> SDWISFSHMSSDTDHFPIKSWFRCEQKAASRSYATLGDMSHPQGIYEVRAAITRLISLTRGVKCRPEQMIIGAGTQVLMQLLTELLPKEAVYAMEEPGYRRMYQLLKNAGKQVKTIMLDEKGMSIAEITRQQPDVLVTTPSHQFPSGTIMPVSRRIQLLNWAAEEPARYIIEDDYDSEFTYDVESIPALQSLDRFQNVIYMGTFSKSLLPGLRISYMVLPPELLRAYKQRGYDLQT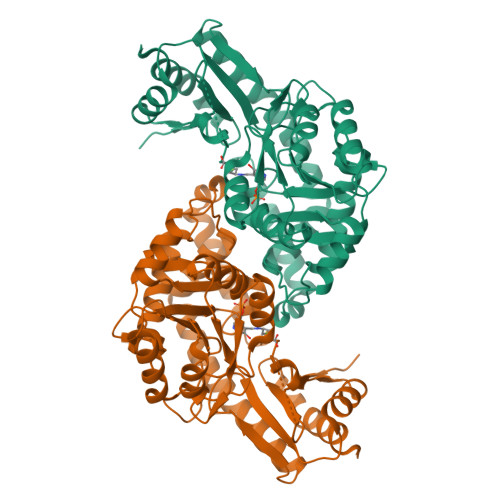CSSLTQLTLQEFIESGEYQKHIKKMKQHYKEKRERLITALEAEFSGEVTVKGANAGLHFVTEFDTRRTEQDILSHAAGLQLEIFGMSRFNLKENKRQTGRPTLIIGFARLKEEDIQEGVQRLFKAVYGH10-DECARBOXYMETHYLACLACINOMYCIN 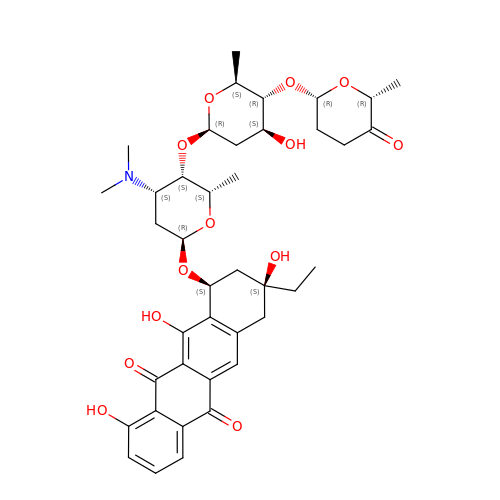A (DCMAA) | C40 H51 N O13 | OXPCRXLITLBLEY-ZVNFQBCFSA-N> MAMYQQYSPKDVVCSWNGIAIEGFAPDSFL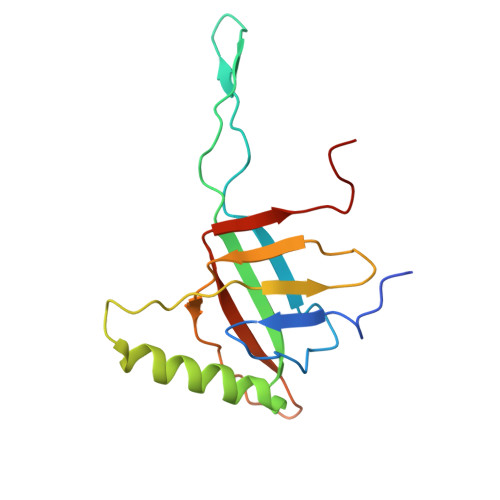RLQRTSPLVTPVVGAGGQVALTRNADKTGTIEIELMQTSLSNQMLSAIQAKQDDMELEEDISSNFVIYDPSGSVLATGINAWLQELPQIELGRDQNSKTWIFGCEKLDYTSTIPASSV> EVARVRNLNRIIMGKYEIEPWYFSPYPIELTDEDFIYIDDFTLQYFGSKKQYERYRKKCTLRHPPGNEIYRDDYVSFFEIDGRKQRTWCRNLCLLSKLFLDHKTLYYDVDPFL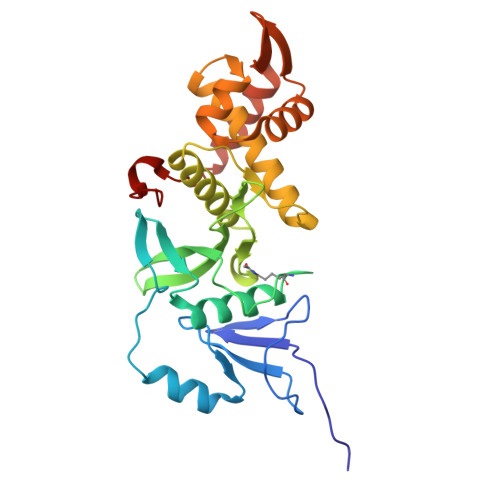FYCMTRRDELGHHLVGYFSKEKESADGYNVACILTLPQYQRMGYGKLLIEFSYELSKKENKVGSPEKPLSDLGLLSYRAYWSDTLITLLVEHQKEITIDEISSMTSMTTTDILHTAKTLNILRYYKGQHIIFLNEDILDRYNRLKAKKRRTIDPNRLIWKPPV>KEWQENKSWNAHFTEHKSQGVVVLWNENKQQGFTNNLKRANQAFLPASTFKIPNSLIALDLGVVKDEHQVFKWDGQTRDIAAWNRDHDLITAMKYSVVPVYQEFARQIGEARMSKMLHAFDYGNEDISGNVDSFWLDGGIRISATQQIAFLRKLYHNKLHVSERSQRIVKQAMLTEANGD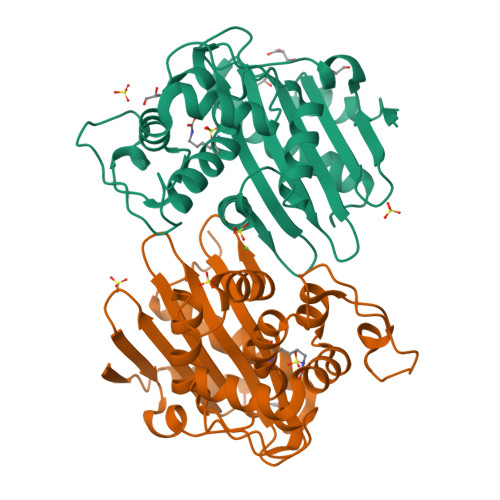YIIRAKTGYSTSIEPKIGWWVGWVELDDNVWFFAMNMDMPTSDGLGLRQAITKEVLKQEKIIPLEH[2x]> KEVKIGMAIDDLRLERWQKDRDIFVKKAESLGAKVFVQSANG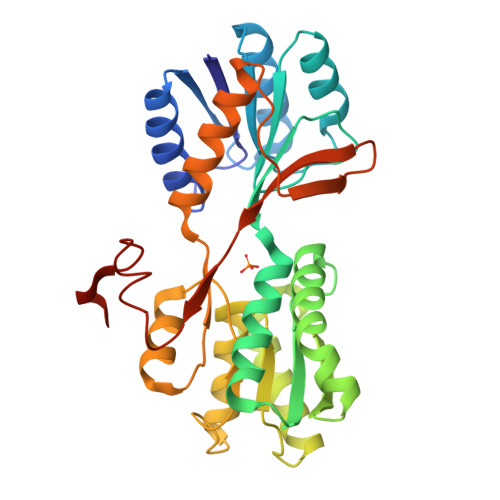NEETQMSQIENMINRGVDVLVIIPYNGQVLSNVVKEAKQEGIKVLAYDRMINDADIDFYISFDNEKVGELQAKALVDIVPQGNYFLMGGSPVDNNAKLFRAGQMKVLKPYVDSGKIKVVGDQWVDGWLPENALKIMENALTANNNKIDAVVASNDATAGGAIQALSAQGLSGKVAISGQDADLAGIKRIAAGTQTMTVYKPITLLANTAAEIAVELGNGQEPKADTTLNNGLKDVPSRLLTPIDVNKNNIKDTVIKDGFHKESELHHHHHH>GSHMSPSDLHLPVPGHPIAAIATPVGVGALAIVRISGAGVLDLADRVFRKVHGSGKLAEAAGYTAHFGRLYDGEEMVDEVIALVFRAPRSFTAEQMVEFTCHGGPVVVGRVLRLMLDNGCRLAEPGEFTRRAFLNGRIDLLQAEAIGEMIHARTESAYRTAVSQMKGDLSVRLGGLREQLIRSCALIELELDFSEEDVEFQSRDELTMQIETLRSEVNRLIDSYQHGRIVSEGVSTVIAGKPNAGKSTLLNTLLGQERAIVSHMPGTTRDYIEECFIHDKTMFR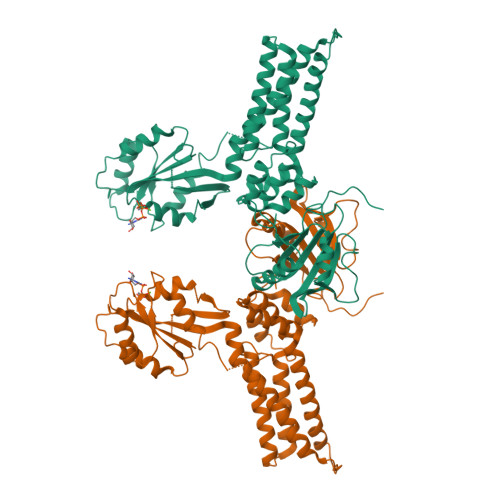LTDTAGLREAGEEIEHEGIRRSRMKMAEADLILYLLDLGTERLDDELTEIRELKAAHPAAKFLTVANKLDRAANADALIRAIADGTGTEVIGISALNGDGIDTLKQHMGDLVKNLDKLHEASVLVTSLRHYEALRNASDALQNALELIAHESETELIAFELRAALDYVGQITGKVVNEEVLNTIFDKFCIGK[3x]> MLAGVKKDIEKLYEAVPQLSNVFKIEDKIGEGTFSSVYLATAQLQVGPEEKIALKHLIPTSHPIRIAAELQCLTVAGGQDNVMGVKYCFRKNDHVVIAMPYLEHESFLDILNSLSFQEVREYMLNLFKALKRIHQFGIVHRDVKPSNFLYNRRLKKYALVDFGLAQGTHDTKIELLKFVQSEAQQERCSQNKPASLTCDCYATDKVCSICLSRRQQVAPRAGTPGFRAPEVLTKCPNQTTAIDMWSAGVIFLSLLSGRYPFYKASDDLTALAQIMTIRGSRETIQAAKTFGKSILCSKEVPAQDLRKLCERLRGAGAGGWNEVPDEAYDLLDKLLDLNPASRITAEEALLHPFFKDMSL;> GPGTRTGRLKKPFVKVEDMSQLYRPFYLQLTNMPFINYSIQKPCSPFDVD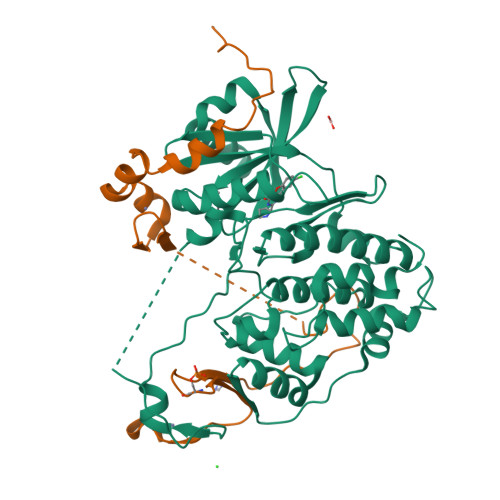KPSSMQKQTQVKLRIQTDGDKYGGTSIQLQLKEKKKKGYCECCLQKYEDLETHLLSEQHRNFAQSNQYQVVDDIVSKLVFDFVEYEKDTPKKKR In an attempt to obtain such “snapshots” of biantennary N-glycan, we selected for crystallographic studies two unrelated plant lectins, Calsepa from Calystegia sepium and PHA-E from Phaseolus vulgaris, which show 4- to 5-fold increase in affinity toward bisected biantennary N-glycans compared with control non-bisected glycan. The most populated conformation of bisected N-glycan is termed the ‘back-fold’ conformation, in which the α1–6 arm is flipped back towards the stem region of N-glycan (GlcNAcβ1–4GlcNAc). In summary, our study provides the first atomic structures of a flipped-back conformation of bisected N-glycan bound to two specific lectins. Thus both proteins, PHA-E as well as Calsepa, are specifically ‘back-fold conformer selective’, rather than broad bisecting GlcNAc-selective lectins.

Calsepa lectin (16 kDa) belongs to mannose-binding type Jacalin-related lectin, and was found to show relatively higher affinity toward bisected glycans than non-bisected glycans. The asymmetric unit contains four Calsepa molecules and two bisected glycans. Two Calsepa molecules sandwich one bisected glycan via an extensive hydrogen bond network as listed in Table S1. In the Calsepa-glycan complex, the α1–6 branch of the glycan is flipped backward (ϕα1–6 = 95, φα1–6 = 105, ωα1–6 = 58) and the conformation is classified as back-fold. Two GlcNAc residues, GlcNAc-5 and GlcNAc-7, are aligned in parallel and the putative hydrogen atoms (H2 and H4) of GlcNAc-7 can make van der Waals contact with the hydrogen atoms (H1, H3 and H5) of GlcNAc-5. In addition, one hydrogen bond is observed between NH group of GlcNAc-5 and N-acetyl carbonyl oxygen atom of GlcNAc-7. The back-fold conformation seems essential to attain the sandwich-like 2:1 interaction. In summary, Calsepa lectin can be considered ‘back-fold conformer selective’, and will not favor a glycan with an extend conformation.

>VPMDTISGPWGNNGGNFWSFRPVNKINQIVISYGGGGNNPIALTFSSTKADGSKDTITVGGGGPDSITGTEMVNIGTDEYLTGISGTFGIYLDNNVLRSITFTTNLKAHGPYGQKVGTPFSSANVVGNEIVGFLGRSGYYVDAIGTYNRHK[4x]>[18x]ATPHINAEMGDFADVVLMPGDPLR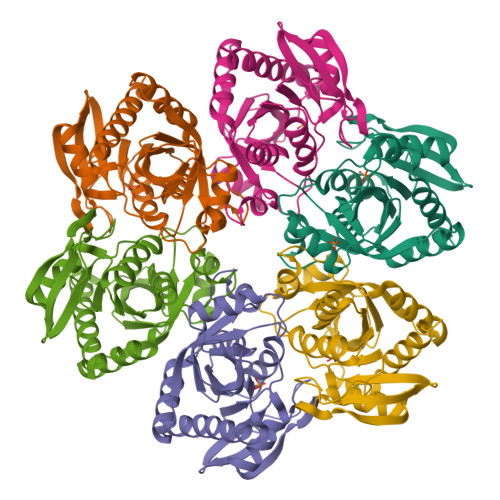AKYIAETFLEDAREVNNVRGMLGFTGTYKGRKISVMGHGMGIPSCSIYTKELITDFGVKKIIRVGSCGAVLPHVKLRDVVIGMGACTDSKVNRIRFKDHDFAAIADFDMVRNAVDAAKALGIDARVGNLFSADLFYSPDGEMFDVMEKYGILGVEMEAAGIYGVAAEFGAKALTICTVSDHIRTHEQTTAAERQTTFNDMIKIALESVLLGDK>[4x]GHHHHHHGSPQRREVAK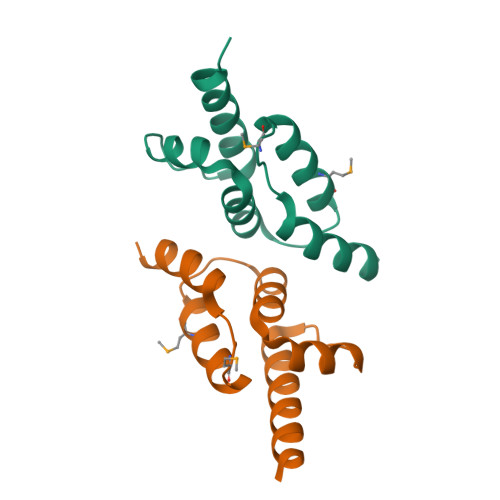RKIRRLRQGMGSVIDYSNAFQMIAQDLDWNEPALIDQYHEGLSDHIQEELSHLEVAKSLSALIGQCIHIERRLARAAAARKPRS> MEVHEEQVSAPVTGDATAKYLLQYILSARGICHENALILALMRLETDASTLNTEWSIQQWVDKLNDYINAINVKLNLLGYKIIRINHGIGRNAVTLKAKQNFESFEDNTAIRAHNNDYAVLQSIVLPESNRFFVYVNLASTEETKLATRFNQNEIEFMKWAIEQFMISGETIVEGPALETSIIVKEVNRILVAATGDSNLAKWRKFSTFTVGSTNLFQFQELTATDIEDLLLRLCELKWFYRTQEGKFG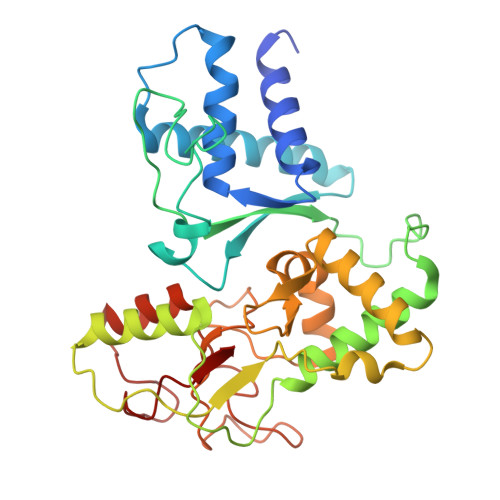IDLRCIAELEEYLTSMYNLNTCQNCHKLAIQGVRCGNESCREENEETGENSLSQIWHVDCFKHYITHVSKNCDRCGSSLITEGVYVI> MALTKAEMSEYLFDKLGLSKRDA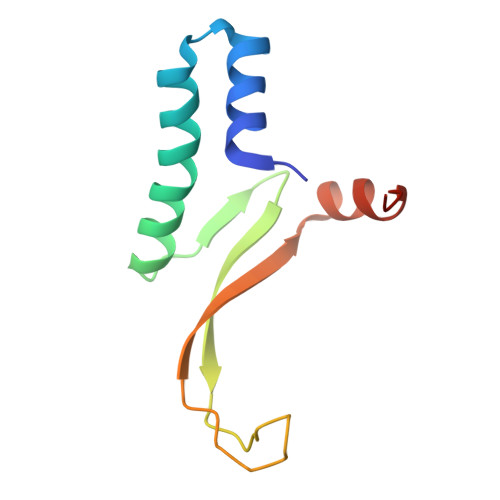KELVELFFEEIRRALENGEQVKLSGFGNFDLRDKNQRPGRNPKTGEDIPITARRVVTFRPGQKLKSRVENASPKDE5-[(1Z)-2-(2-methoxyphenyl)-3-methylbut-1-en-1-yl]furo[2,3-d]pyrimidine-2,4-diamine | C18 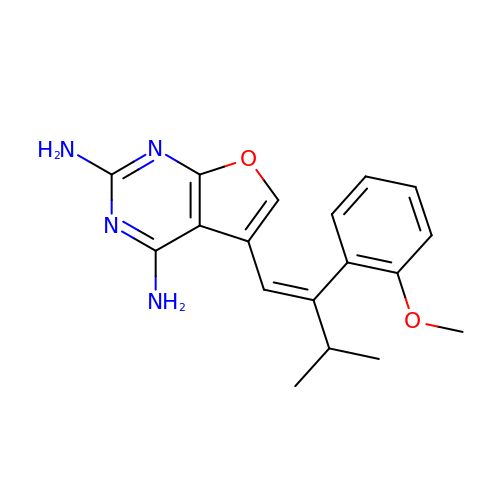H20 N4 O2 | ZBHMLBFDTQKTKI-JYRVWZFOSA-N>GSHNSHMKLQEVEIRNKDLEGQLSEMEQRLEKSQSEQDAFRSNLK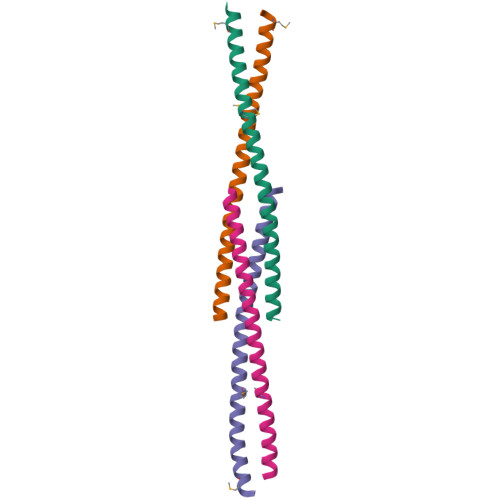TLLEILDGKIFELTELRDNLAKLLECS[4x]> STQNSSSVQDKQLQKVEEVPNNSEKALVKKLYDRYSKDTINGKSNKSRNWVYSERPLNENQVRIHLEGTYTVAGRVYTPKRNITLNKEVVTLKELDHIIRFAHISYGLYMGEHLPKGNIVINTKNGGKYTLESHKELQKNRENVEINTDDIKNVTFELVKSVNDIEQV

The superantigenic properties of Staphylococcal enterotoxin-like X (SElX) have recently been established. We now reveal that SElX also possesses functional characteristics of the SSLs. Here we present functional and structural evidence that SElX is an ‘SSL-like’ SAg. It has specificity for sLacNac and interacts with myeloid cells in a sialylated glycan-dependent manner to inhibit host defences. Consequently, SElX targets both the adaptive immune system as a SAg and innate immune defences as an SSL.

The crystal structure of SEIX8 was determined in complex with sLeX. The C-terminal domain of SEIX8 (residues N61–I161) adopts the β-grasp fold typical of the classical SAgs and members of the SSL family. The first 21 residues and the last 3 residues of the mature protein were undefined in the crystal structure, lacking electron density. The first structured residue N22 defines the start of the α-helix that sits atop the rear of the β-grasp C-terminal domain. An extended loop, which is stabilized by extensive hydrogen bonds, links the bottom of this helix directly with the first β strand of the β-grasp domain. It completely replaces the typical OB-fold domain, revealing SElX to be a unique single-domain SAg. The binding site for sLeX is a V-shaped depression in the side of the β-grasp domain, which is formed by residues from a β-strand, the opposing helix (a 310-helix), and the irregular polypeptide loop that links them. Seven residues lining the sides of the depression hydrogen bond directly to sLeX. These are the side-chains of T130, E132, K135, Q138, N140, and R141, and the main chain carbonyl of K128. Indeed, the binding of sLeX is almost entirely conserved with the sLeX binding of SSL4, SSL5, and SSL11.>MADSSEGPRAGPGEVAELPGDESGTPGGEAFPLSSLANLFEGEDGSLSPSPADASRPAGPGDGRPNLRMKFQGAFRKGVPNPIDLLESTLYESSVVPGPKKAPMDSLFDYGTYRHHSSDNKRWRKKIIEKQPQSPKAPAPQPPPILKVFNRPILFDIVSRGSTADLDGLLPFLLTHKKRLTDEEFREPSTGKTCLPKALLNLSNGRNDTIPVLLDIAERTGNMREFINSPFRDIYYRGQTALHIAIERRCKHYVELLVAQGADVHAQARGRFFQPKDEGGYFYFGELPLSLAACTNQPHIVNYLTENPHKKADMRRQDSRGNTVLHALVAIADNTRENTKFVTKMYDLLLLKCARLFPDSNLEAVLNNDGLSPLMMAAKTGKIGIFQHIIRREVTDEDTRHLSRKFKDWAYGPVYSSLYDLSSLDTCGEEASVLEILVYNSKIENRHEMLAVEPINELLRDKWRKFGAVSFYINVVSYLCAMVIFTLTAYYQPLEGTPPYPYRTTVDYLRLAGEVITLFTGVLFFFTNIKDLFMKKCPGVNSLFIDGSFQLLYFIYSVLVIVSAALYLAGIEAYLAVMVFALVLGWMNALYFTRGLKLTGTYSIMIQKILFKDLFRFLLVYLLFMIGYASALVSLLNPCANMKVCNEDQTNCTVPTYPSCRDSETFSTFLLDLFKLTIGMGDLEMLSSTKYPVVFIILLVTYIILTFVLLLNMLIALMGETVGQVSKESKHIWKLQWATTILDIERSFPVFLRKAFRSGEMVTVGKSSDGTPDRRWCFRVDEVNWSHWNQNLGIINEDPGKNETYQYYGFSHTVGRLRRDRWSSVVPRVVELNKNSNPDEVVVPLDSMGNPRCDGHQQGYPRKWRTDDAPLENSLEVLFQGPDYKDDDDKAHHHHHHHHHH[4x]

TRPV4 is a polymodal, calcium-permeable cation channel that has emerged as a potential therapeutic target in multiple conditions. TRPV4, expressed in the plasma membrane of a wide range of cell types, is a polymodal ion channel whose gating is controlled by multiple endogenous lipids, and exogenous stimuli including synthetic ligands, cell swelling, shear stress, moderate heat, and ultraviolet light. Human TRPV4 adopts a two-layered homotetrameric architecture where RhoA attaches to the bottom layer. RhoA appears to act as an auxiliary subunit, interacting with the ARD through three loops connecting AR2-AR3, AR3-AR4, AR4-AR5, and with the membrane bilayer through the prenylated C-terminal tail.

Three additional complex structures were determined in the presence of distinct ligands: the antagonist GSK2798745-bound TRPV4-RhoA complex in the closed state, the agonist GSK1016790A-bound TRPV4-RhoA in the open state, and the agonist 4α-phorbol 12,13-didecanoate-bound TRPV4-RhoA in the putative open state (ligands are abbreviated as GSK279, GSK101, and 4α–PDD, respectively). In our ligand-bound 3D cryo-EM reconstructions, we identified strong and unambiguous EM densities corresponding to GSK279 (antagonist), GSK101 (agonist), and 4α-PDD (agonist) located at a shared site within the cavity between the VSLD and the TRP domain (termed here the VSLD cavity). For 4α−PDD binding poses, we tested three poses, and pose III remains relatively stable while the other two poses are dynamic, supporting that pose III is likely the binding mode of 4α-PDD to TRPV4. Although the EM density for the pore domain in the ligand-free state and the 4α-PDD-bound structures was resolved sub-optimally, the high-quality reconstructions for the GSK279-bound closed state and the GSK101-bound open state enabled us to unambiguously model the register and assign the gate residues.>[2x]GPGSISLGDLHGNAIKLIHFLFRHKIIKFKTEIINFHEAYQQFVTIYEQYDDMVQEYLEIRTLLQLIQIKITNAQQRILDIEQKLSLATDHQKEFSQSLLQLKKPIEANLQMAEKSKAGLEEKLSGLKTRLPSCIERFNKFMTQIEINDIKTLIRLLGDEVADRGSCDYFTLRILDFLYQNQIAIKIILSNHGYEFIHAYEKLVVGQPFKPKGYIGDIQIKSFWGLQLLLEQSVITEEELRSLVERAYKPTLKIIDYSLSEDGITLYSHAPIRFDSIRMAASQLGVTYNDSTKEALAETIDQLNAQLQIYMKNNMLHLLFENNEINDPTNMTDEERNASPLIYLVWNRWNESKEVENARPGKYNGYFVTYVHGHDPFQSPLTYVYNLDTLCGKYSRVGEEEQINKAFQFLTENR

Here we describe the crystal structure and biochemical properties of WipA (or IcmW-interacting protein A; lpg2718), an effector protein originally identified because of its dependence on the IcmSW complex for translocation, but for which the function is unknown. The crystal structure reveals a two-domain structure comprising a metallophosphoesterase attached to an 85-Å-long α-helical hairpin forming a coiled-coil at its tip. Although WipA exhibits a serine/threonine phosphatase fold, it functions preferentially as a protein-tyrosine phosphatase (PTP), even though there are no structural similarities to the general PTP fold. The protein forms homodimers in solution, and the dimer is mediated by the tip of the helical hairpin domain.

Subsequently, a larger fragment, from residue 24 to residue 435 (termed “WipA435”) was produced containing a more complete active site. WipA435 crystallized in the presence of MnCl2 and crystals diffracted to a resolution of 1.75 Å. The WipA435 structure was determined by molecular replacement using the WipA411 structure as a search model. The model of WipA435 contains residues 24–418 in one molecule and residues 24–422 in the other. The two protomers of WipA435 superimpose with each other with an RMSD value of 0.72 Å, suggesting identical structures. The second interface is observed only in the WipA435 crystals and involves a disulfide bridge from Cys412 and a Mn2+ ion coordinating two Asp409 residues from symmetrically related molecules. A difference anomalous Fourier map revealed the presence of four Mn2+ ions: one in each molecule refined to full occupancy that appear strongly bound, two (one at the interface between two WipA molecules, and one in chain B in the proximity of the active site) appearing to be weakly bound. The strongly bound ions locate within proximity of three sequence motifs (DXH, GDXXDR, and GNHE) known to be signature motifs for metallophosphoesterases, suggesting that these ions (one in each protomer) might be catalytic ions and that the residues around them might form the active site. All three sequences in the structure locate in one region of the structure, suggesting that the active site of WipA is located there. This region indeed comprises the one fully occupied Mn2+ cation described above in a tetrahedral bipyramidal arrangement coordinated by the WipA residues Asp180, His290 (a residue outside the phosphatase motifs), and Asn212, two water molecules, and a phosphate ion. The fact that we do not observe Mn2+ bound to His32 might be due to an incomplete structure lacking a large part of the C terminus of the full-length protein. This is consistent with WipA435 being inactive in the phosphatase assay (data not shown).> AGHMSDAKATAGSEPEAEPLTKRLSKASRKIHNVSNSLVNARLIALFSDKDLYAKALGCFYYVFVALEAALDEALKKGDADVSKFKDVLKGGLYRAPGFKQDVQHYLGATWQAQLGTKSQALKDYEAHLASLGRSSPALLLAHVYTQHLAMASGGQIVKRWARKIFQLPDDVG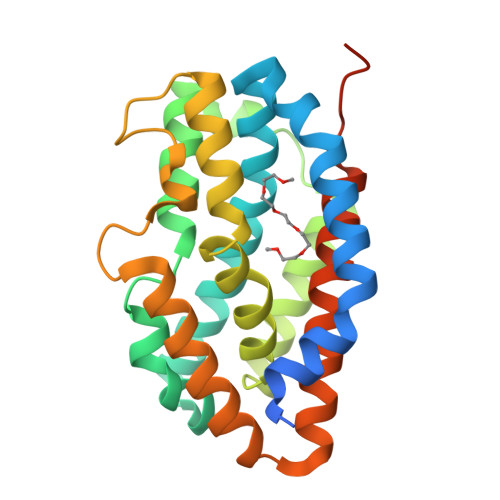TAAFDYTGESNNTLRSAFKKQFDEWGAAQPQELQDQLLSEHLAAFGHNNAIIKAFPLPATAIIAGAIRVTPRPG N-{3-[(8-phenyl[1,2,4]triazolo[1,5-a]pyridin-2-yl)amino]phenyl}propanamide 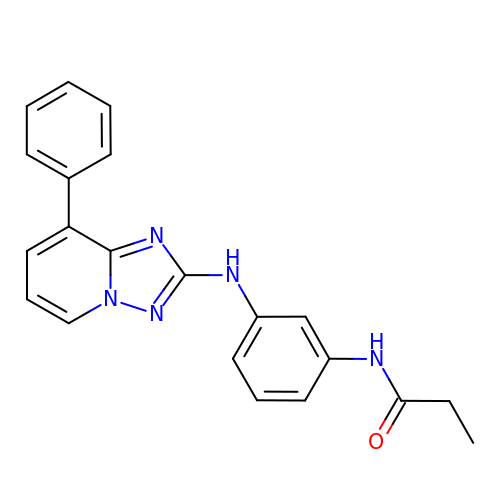| C21 H19 N5 O | LFWOSNJNBDQUPD-UHFFFAOYSA-N>[4x]GAGTMVKQIESKTAFQ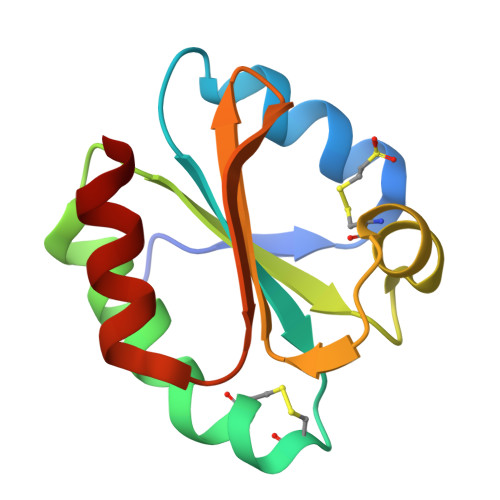KALKAAGDKLVVVDFSATWCGPCKMIKPFFHSLSEKYSNVIFLEVDVDDCQDVASECEVKCMPTFQFFKKGQKVGEFSGANKKKLEATINKLV>MAFMKKYLLPILGLFMAYYYYSANEEFRPEMLQGKKVIVTGASKGIGREMAYHLAKMGAHVVVTARSKETLQKVVSHCLELGAASAHYIAGTMEDMTFAEQFVAQAGKLMG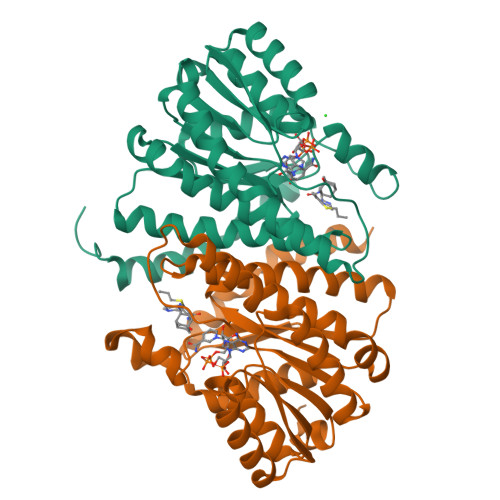GLDMLILNHITNTSLNLFHDDIHHVRKSMEVNFLSYVVLTVAALPMLKQSNGSIVVVSSLAGKVAYPLVAAYSASKFALDGFFSSIRKEYSVSRVNVSITLCVLGLIDTETAMKAVSGIVHMQAAPKEECALEIIKGGALRQEEVYYDSSRWTTLLIRNPSRKILEELYSTSYNWDRFINK[2x]We first show that S-Cys-Gly-3M3SH is actively taken up by S. hominis through a specific secondary active transporter, STAH0001_1446 (SH1446), a member of the proton coupled oligopeptide transporter (POT) family. POT transporters belong to the Major Facilitator Superfamily (MFS) and use an inwardly directed proton electrochemical gradient to drive the concentrative uptake of di- and tri-peptides across the cell membrane for metabolic assimilation. We and others have demonstrated that S-Cys-Gly-3M3SH can be taken up and metabolised by a highly limited range of staphylococcal species present in the axilla, namely Staphylococcus hominis, Staphylococcus haemolyticus and Staphylocooccus lugdunensis, to liberate 3M3SH, that subsequently exits the cell through an undefined mechanism. While S-Cys-Gly-3M3SH is a highly modified and uniquely human dipeptide, we reasoned that this moiety might dictate the uptake mechanism into malodour producing bacteria and here we identify a peptide transporter, PepTSh (SH1446), from the POT family of secondary active transporters as being responsible for this process.

To gain further insight into the mechanism of substrate binding we successfully obtained a high-resolution co-crystal structure of PepTSh at 2.5 Å resolution, bound to S-Cys-Gly-3M3SH using the in meso crystallisation method. PepTSh adopts the canonical MFS fold with helices H1-H6 forming the N-terminal bundle and H7-H12 the C-terminal bundle. PepTSh was crystallised in an inward open state, observed previously for other members of the POT family, wherein the extracellular gate, consisting of helices H1-2 and H7-8 from the N- and C-terminal bundles respectively, is closed and the intracellular gate, consisting of helices H4-5 and H10-11 is open. Unlike previous POT structures however, PepTSh also contains a well-structured β-hairpin motif between helices H7 and H8 on the extracellular side of the membrane, extending out in line with the lipid head groups. Interestingly we observed a number of monoolein lipid molecules that cluster around both the β- hairpin and the cavity created between helices HA and HB with the transporter domain. The Cys-Gly part of the precursor is positioned such that the carboxy termini of the peptide faces towards the intracellular side of the binding site. The terminal carboxyl group makes two hydrogen bond interactions, one with Tyr41 on H1 and a second interaction to a water molecule (W107), which links the carboxyl group with Asn347 on H8. The carbonyl group of the CG peptide also makes a hydrogen bond to this water molecule, creating a well-coordinated interaction network between the peptide and Asn347. The terminal amino group makes two further polar interactions, with a water molecule that sits next to Tyr41 and also to the carbonyl group of Gln344, which sits further up on H8.

> QTIQSIPQKGFFGHPRGLGVLFFVEFWERFSYYGMRAMLIFYMYFAIHQNGLGIDKTTAMSIMSVYGALIYMSSIPGAWIADRITGTRGATLLGAVLIIIGHICLSLPFALFGLFSSMFFIIIGSGLMKPNISNIVGRLYPENDTRIDAGFVIFYMSVNLGALISPIILQHFVDIRNFHGGFLLAAIGMALGLVWYLLFNRKNLGSVGMAPTNPLSKEEKRKYGMIIGIIVAIVIVVLLVTYYTHTLSFDLISNTVLVLGVALPIIYFTTMLRSKDVTDGERSRVKAFIPLFILGMLFWSIQEQGSNVLNIYGLERSDMQLNLFGWTTRFGEALFQSINPLFILLFAPVISMIWLKMGKKQPSLAIKFSIGTLLAGLSYILIGLVGLGYGHTQFSVNWVILSYVICVIGELCLSPTGNSAAVKLAPKAFNAQMMSVWLLTNASAQAINGTLVKLIKPLGQTNYFIFLGTVAIVITLIILVFSPKITK> ALLDETPLPPGSRLDVRAYTTVLHALSRAGRYERALELFAELRRQGVAPTVVTYNTLIDGLCKAGKLDEALKLFEEMVEKGIKPDVVTYNTLIDGLCKAGKLDEALKLFEEMVEKGIKPDVVTYNTLIDGLCKAGKLDEALKLFEEMVEKGIKPDVVTYNTLIDGLCKAGKLDEALKLFEEMVEKGIKPDVVTYSTLIDGLCKAGKLDEALKLFEEMVEKGIKPNVVTYSTLIDGLCKAGKLDEALKLFEEMVEKGIKPNVVTYNTLIDGLCKAGKLDEALKLFEEMVEKGIKPDVVTYNTLIDGLCKAGKLDEALKLFEEMVEKGIKPDVVTYNTLIDGLCKAGKLDEALKLFEEMVEKGIKPDVVTYNTLIDGLCKAGKLDEALKLFEEMVEKGIKPDELTYRRVVESYCRAKRFEEARGFLSEVSETDLDFDKKALEAYIEDAQFGRLEHHHHHHHH

Containing a tandem array of 2–30 repeats, pentatricopeptide repeat (PPR) proteins constitute one of the largest protein families in land plants. Each PPR repeat aligns to a single nucleotide of the RNA target in modular patterns, making these proteins suitable for the development of exciting new biotechnologies. Within each repeat, the combinations of two amino acids, known as the PPR code at two key positions (the 5th and the 35th) confer RNA specificity. A typical RNA-bound dPPR protein adopts a right-handed superhelical spiral structure, with its target ssRNA molecule sitting in the interior cavity and interacting with corresponding PPR repeats in a modular fashion.

To verify the RNA selectivity, the dPPR proteins dPPR-U8N2 (in which N indicates any nucleotide) comprising 10 dPPR repeats with different 5th and 6th repeats with different PPR codes were constructed and purified to homogeneity. After numerous unsuccessful trials, we finally succeeded in crystallizing each dPPR-U8N2 in complex with its respective target ssRNA (5′-UUUUNNUUUU-3′), in space group P212121. When dPPR-U8C2 was superimposed on dPPR-U10, dPPR-U8A2 and dPPR-U8G2, the root mean square deviations were 0.73, 0.99 and 1.00 Å over 348, 367 and 374 Cα atoms, respectively. As observed in all four complex structures, four types of dPPR repeats recognize their corresponding targets by forming hydrogen bonds with the Watson–Crick faces of the nucleotides, which explains why PPR proteins bind ssRNAs instead of double stranded ones. Serine or threonine at this position results in a preference for purines, whereas the presence of asparagine is correlated with a preference for pyrimidines. The amide group of the Asn5 side chain donates a hydrogen bond to the O2 atom of the corresponding pyrimidine, whereas the N3 atom of purine accepts a hydrogen bond from the hydroxyl group of the corresponding amino acid. For purine, Asn35 or Asp35 form one or two hydrogen bonds with adenine and guanine, respectively. The N1 atom of adenine is a hydrogen bond acceptor, whereas both the N1 and N2 atoms of guanine are hydrogen bond donors. These structures demonstrate how the amino acids asparagine and aspartate at the 35th position contribute to purine base selectivity.>SNAMYLRRFYDEGLAHASYLVGCQETGEACVIDPARDVEPYLLTAKREGLRIVAALETHIHADFVSGAREMADRAGAAICVSDEGPPEWKSEYVKAYPHRLLKDGDELHFGNVRIVVMHTPGHTPEHVSYLLYDGKTSPDVP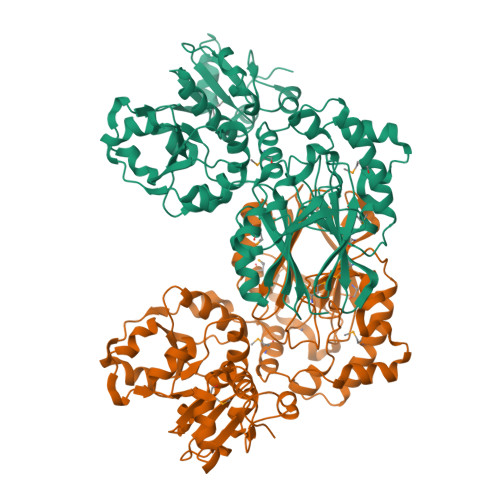MALFSGDFVFVGDVGRPDLLERVAGESGSSEALARQMFRSLRKFEALPDHVQVLPAHGAGSACGKALGAVPSSTVGYEKLVNWALQHKDEDAFVQALLAGQPEAPIYFARMKLVNKVGPRLLAELGAPERVDLPPERVRAWREGGVVLDVRPADAFAKRHLAGSLNIPWNKSFVTWAGWLLPADRPIHLLAADAIAPDVIRALRSIGIDDVVDWTDPAAVDRAAPDDVASYANVSPDEVRGALAQQGLWLLDVRNVDEWAGGHLPQAHHIPLSKLAAHIHDVPRDGSVCVYCRTGGRSAIAASLLRAHGVGDVRNMVGGYEAWRGKGFPVEA[2x]>MAHHHHHHSSGLEVLFQGPMTHSVVELIEIESAIIQVKMQDRTHKNAFSQELTDDLIQAFEYIRQNPKYKAVILTGYDNYFASGGTQEGL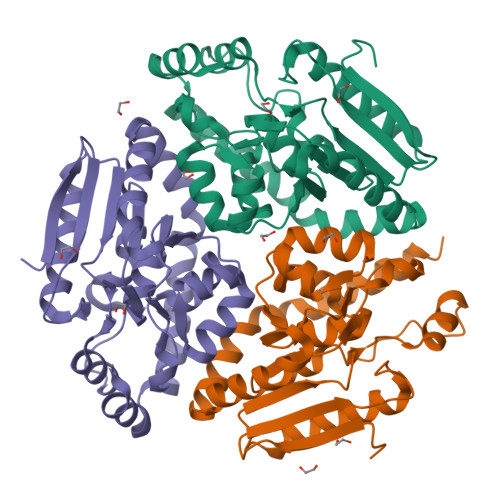LRIQQGLTKFTDDNLYSLALDCEIPVIAAMQGHGIGGGFVMGLFADIVILSRESVYTANFMKYGFTPGMGATFIVPKKLGFSLAQEILLNAGSYRGADLEKRGVPFKVLPRAEVLDYAVELAQELAEKPRNSLVTLKDHLVAPLRDQLPRVIEQELMMAEKTFHHEEVKSRIKGLYGN[3x]2,4-DICHLORO-6-(3,4,5-TRIBROMO-1H-PYRROL-2-YL)PHENOL 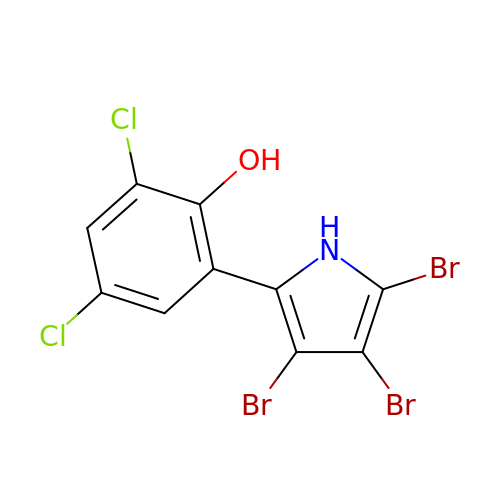| C10 H4 Br3 Cl2 N O | KMUJMUQZYHMNDR-UHFFFAOYSA-N> DVGEEFNQEAEYGGHDQIDLYDDVISPSANNGDAPEDRDYMDTLPPTVGDDVGKGAAPNVVYTYTGKRIALYIGNLTWWTTDEDLTEAVHSLGVNDILEIKFFENRANGQS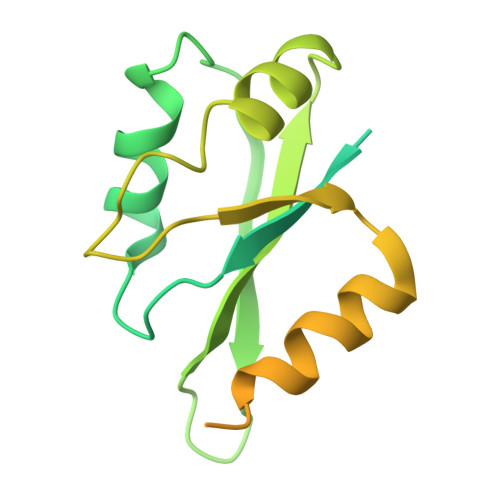KGFALVGVGSEASSKKLMDLLPKRELHGQNPVVTPVNKQFLSQFEMQSRKTTQSGQMSGEGKAGPPGGSSRAAFPQGGRGRGRFPGAVPGGDRFPGPAGPGGPPPPFPAGQTHHHHHH> MGFEFTLMVVGESGLGKSTLINSLFLTDLYPERVIPGAAEKIERTVQIEASTVEIEERGVKLRLTVVDTPGYGDAINCRDCFKTIISYIDEQFERYLHDESGLNRRHIIDNRVHCCFYFISPFGHGLKPLDVAFMKAIHNKVNIVPVIAKADTLTLKERERLKKRILDEIEEHNIKIYHL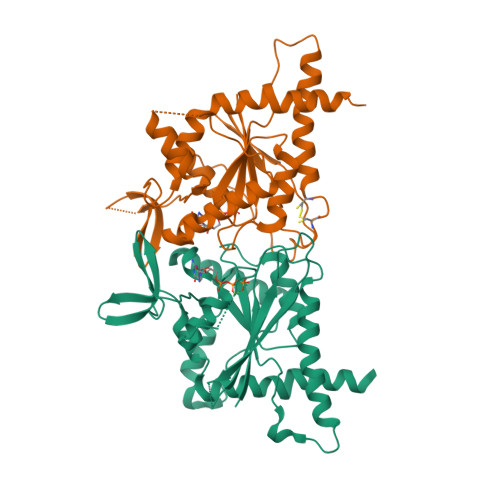PDAESDEDEDFKEQTRLLKASIPFSVVGSNQLIEAKGKKVRGRLYPWGVVEVENPEHNDFLKLRTMLITHMQDLQEVTQDLHYENFRSERLKRGGLESGKETAAAKFERNHMDSSTSAA;> MGSSHHHHHHSQDPGFCFNILCVGETGLGKSTLMDTLFNTKFEGEPATHTQPGVQLQSNTYDLQESNVRLKLTIVSTVGFGDQINKEDSYKPIVEFIDAQFEAYLQEELKIRRVLHTYHDSRIHVCLYFIAPTGHSLKSLDLVTMKKLDSKVNIIPIIAKADAISKSELTKFKIKITSELVSNGVQIYQFPTDDESVAEINGTMNAHLPFAVIGSTEELKIGNKMMRARQYPWGTVQVENEAHCDFVKLREMLIRVNMEDLREQTHTRHYELYRRCKLEE> MKIIKDKVAKLSFVALLVTVTAAMFYTPTASA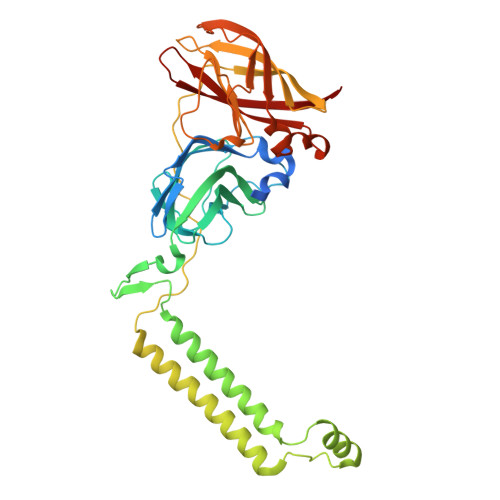HGEKSQAAFMRMRTIHWFDLNWSKDQVSVNETMSISGKFHVFAGWPETVDKPEVAFLNIGIPGPVFIRAGSWIGGQLVPRSVSLELGETYEFKVLLKARRPGDWHVHTMMNVQGGGPIIGPGKWVTITGSMGDFKNPITTLTGETIDLETYALDGVYGWHLFWYLLGVAWMVYWCRKPVFIPRRIAVDAGKADSLITPTDKKVGMAFAAGTLAIVAVSMGQANEKYPVTTPLQAGLMRGIKSLELPQPTVSVKVVDASYRVPGRAMQMTLEITNNGDSAVRLAEFNTASVRFLDADVYEDDTNYPDDLLAEEGLSVSDNSPLAPGETRTVDVTASDAAWEVYRLADLIYDPDSRFAGLLFFIDEDGNRQMTMVDAPLIPTFI>MSTSGTGKMTRAQRRAAARRNRWTARVQPVIVEPLAAGQGKAIKAIAGYSISKWEASSDAITAKATNAMSITLPHELSSEKNKELKVGRVLLWLGLLPSVAGRIKACVAEKQAQAEAAFQVALAVADSSKEVVAAMYTDAFRGATLGDLLNLQIYLYASEAVPAKAVVVHLEVEHVRPTFDDFFTPVY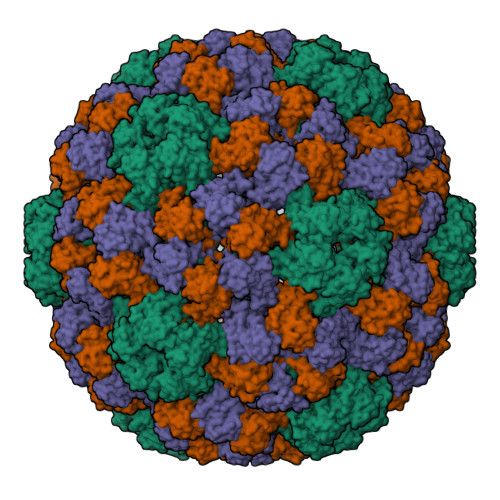R[3x]>GSPVVVGSKPAQRFAVLYGTMCDILNGYDNQVVMQQKLKEFIEVLRDPKLPYSEFSAQFSALHARMPHKLDAQLTQVLERAQNRGAEFPARQLLKVFNKFLDDNVPNKTDQDLLKSTLEPLTSVLNLYLDGQKARELNLIADLLSMYADVECQFSGRRLQDEEAILKLRDQYKDNIQKVVNTVLSHKNVMSKNSLVLALLDEYRPNKPNVGNVGKHLRPVLRRLTELESRQSAKVSLKAREVLILCALPSLEERTAQMEHILRSSVVQSRYGETGWSHRRPDREVLKEVVDSKYTVFDVLTLFFAHEDPYVALAALEVYVRRAYRAYNLREVRYHDEERPYFIDWDFALRKSGANQTESSMHMQSVVPSSPATPVENDFKRIHSISDMTYLARRTRDEPIRKGVIVPCKDLLDAEEALSRALEVLPLAHKETKDKDRKQQPGIAADLAQRRRPGTPLRLEGIGELSAVVNVAVRDAEGKNDEEILALIKPWVQNSKADLLARRVRRLTFICGRNDGSYPSYYTFRGPDYAEDDSIRHIEPSLAFQLELGRLSKFKLTPVFTQNKNIHVYEAVGRGVETDRRYFTRAVVRPGRLRDEISTAEYLISEADRVVNDIFDALEIIGTNKTDLNHMFINFSHTFQVTADEVAESLQGFLDRFGPRGWRLRVHQVEIRINCMRSDNNDENDTMPLRVIITNTSGFVIQIELYEEKLSEKGEWVYYYVSGNAKIGSMHLLPVSTPYPTKNWLQPKRYKAHILGTQYVYDFPELFRQAIQNSWTEAVKKIPSLAAKQPAIGECIDYNELVLGDQDNLAEVSREPGMNSTGMVGWLINARTPEYPDGRKFIVVANDITFKIGSFGPKEDTFFFKCTELARKMGIPRIYLSANSGARLGLAEELMPHFNVAWNDPAKPEAGFKYLYLSDEAKRRFENEVITEEIVEDGEKRHKIITIVGAEEGLGVECLRGSGLIAGATSRAYNDIFTCTLVTCRSVGIGAYLVRLGQRAVQVEGQPIILTGAPALNSLLGREVYTSNLQLGGTQIMYRNGVSHLTAKDDFDGVTKIVQWLSFIPDQRNNPLPILSPSPDPWDRDVVYTPPYKQTYDVRWMIAGKEDEDGFQPGLFDKDSFVETLGGWARTVVVGRARLGGIPMGVIAVETRTIENITPADPANPDSIEQVTNEAGGVWYPNSAFKTAQAINDFNYGEQLPLMILANWRGFSGGQRDMYNEVLKYGSFIVDALTRFEKPIFIYIPPH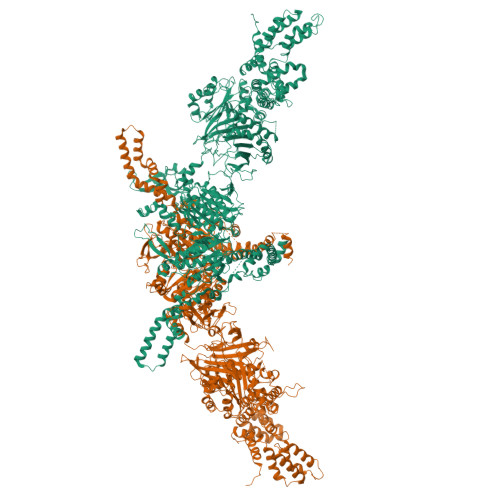GELRGGSWVVVDPTINPASMEMYADEEARGGVLEPEGIIPIKYKKDKQLETMARLDPVYRSLKKEMAKEGLSKEESDNIKKKMQQREELLLPIYHQICVQFADLHDRAGRMKAKGVIRQSLQWRQSRRFFYWRVRRRLIEDDILRRIEEAINPAGKRRHDPENTSLAASPETRSPHLVQLESWVGIPGFKTNDREVVEWYEQNQDRINEKLEKLKKESIADQMRELLRXXXXXXXXXXXX[2x]>MDLTHFQDGRPRMVDVTEKPETFRTATAEAFVELTEEALSALEKGGVGKGDPLVVAQLAGILAAKKTADLIPLCHPLPLTGVEVRVELLKAEKRVRIEATVKTKAETGVEMEAMTACAVAALTVYDMLKAASKGLVISQVRLL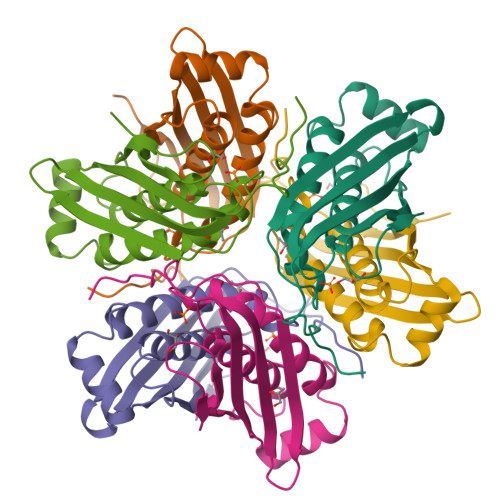HKAGGKSGEWRREQ[12x]The envelope glycoprotein B (gB) is a major viral antigen known to play a crucial role in PRV entry. As the viral fusogen, gB is essential for both viral entry and cell-to-cell spread. In this work, we immunized mice with soluble PRV gB to generate gB specific mAbs and identified a total of 15 neutralizing antibodies that effectively block PRV entry with either complement dependent or independent mechanisms.

Thus, we recombinantly expressed a truncated PRV gB protein, denoted as PRV gB-D_IV, which includes the domain IV and a portion of the adjacent domain III central helix. Based on the ELISA experiments, all the 14 complement-dependent neutralizing antibodies can bind to both gB and gB-D_IV, indicating the epitopes of these antibodies are very probably within the domain IV of gB. In order to further characterize the immunogenic properties of PRV gB and identify the epitopes of these neutralizing antibodies, we determined the crystal structures of PRV gB and gB-D_IV at 3.1 and 2.7 Å resolution, respectively. Domain IV wraps around the top of the central helix bundle to form a crown in the bottle-shaped gB trimer. The trimerization interfaces are highly stable, such that the truncated gB-D_IV could also assemble into trimers. The structure of gB-D_IV trimer could be ideally superimposed with the corresponding portion in the context of the entire gB ectodomain, with a rmsd of 0.598 Å. The highly stable structure of gB-D_IV further supported the conclusion from our ELISA based assays that these complement-dependent neutralizing antibodies target the crown region of PRV gB and very probably within domain IV. Based on the gB structure we present in this study, domain IV is located on the apexes of the gB trimer to form a "crown", making it fully accessible for both antibody and potential receptor recognition. However, all the antibodies targeting domain IV of gB reported to date do not directly block PRV entry but dependent on the complement effect instead, as shown by cell-based assays in vitro. This phenomenon implies that domain IV is probably not a receptor binding site for PRV gB, and that it might retain the same fold before and after membrane fusion with only domain rearrangement in the process of gB conformational changes to mediate membrane fusion.

>TRAASASPAPGTGATPDGFSAEESLEEIDGAVSPGPSDAPDGEYGDLDARTAVRAAATERDRFYVCPPPSGSTVVRLEPEQACPEYSGGSGNDMLSRIAAAWCELQNKDRTLWGEMSRLNPSAVATAALGQRVSARMLGDVMAISRCVEVRGGVYVQNSMRVPGERGTCYSRPLVTFEHNGTGVIEGQLGDDNELLISRDLIEPCTGNHRRYFKLGGGYVYYEDYSYVRMVEVPETISTRVTLNLTHHHHHHHH[6x]> HLEVVK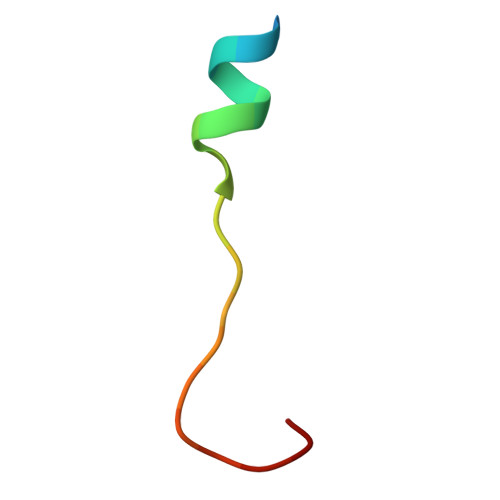LLLEHGADVDAQDK> MDPPRPALLALLALPALLLLLLAGARAEEEMLENVSLVCPKDATRFKHLRKYTYNYEAESSSGVPGTADSRSATRINCKVELEVPQLCSFILKTSQCTLKEVYGFNPEGKALLKKTKNSEEFAAAMSRYELKLAIPEGKQVFLYPEKDEPTYILNIKRGIISALLVPPETEEAKQVLFLDTVYGNCSTHFTVKTRKGNVATEISTERDLGQCDRFKPIRTGISPLALIKGMTRPLSTLISSSQSCQYTLDAKRKHVAEAICKEQHLFLPFSYKNKYGMVAQVTQTLKLEDTPKINSRFFGEGTKKMGLAFESTKSTSPPKQAEAVLKTLQELKKLTISEQNIQRANLFNKLVTELRGLSDEAVTSLLPQLIEVSSPITLQALVQCGQPQCSTHILQWLKRVH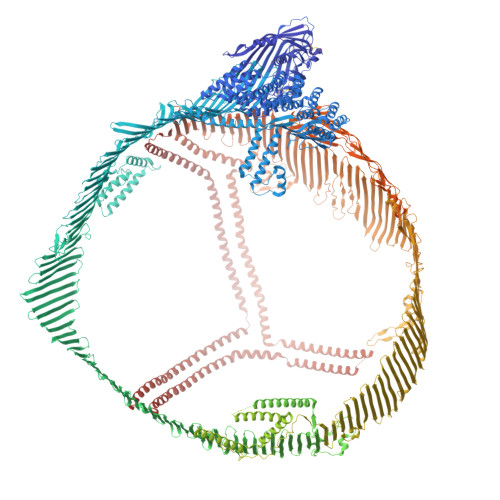ANPLLIDVVTYLVALIPEPSAQQLREIFNMARDQRSRATLYALSHAVNNYHKTNPTGTQELLDIANYLMEQIQDDCTGDEDYTYLILRVIGNMGQTMEQLTPELKSSILKCVQSTKPSLMIQKAAIQALRKMEPKDKDQEVLLQTFLDDASPGDKRLAAYLMLMRSPSQADINKIVQILPWEQNEQVKNFVASHIANILNSEELDIQDLKKLVKEALKESQLPTVMDFRKFSRNYQLYKSVSLPSLDPASAKIEGNLIFDPNNYLPKESMLKTTLTAFGFASADLIEIGLEGKGFEPTLEALFGKQGFFPDSVNKALYWVNGQVPDGVSKVLVDHFGYTKDDKHEQDMVNGIMLSVEKLIKDLKSKEVPEARAYLRILGEELGFASLHDLQLLGKLLLMGARTLQGIPQMIGEVIRKGSKNDFFLHYIFMENAFELPTGAGLQLQISSSGVIAPGAKAGVKLEVANMQAELVAKPSVSVEFVTNMGIIIPDFARSGVQMNTNFFHESGLEAHVALKAGKLKFIIPSPKRPVKLLSGGNTLHLVSTTKTEVIPPLIENRQSWSVCKQVFPGLNYCTSGAYSNASSTDSASYYPLTGDTRLELELRPTGEIEQYSVSATYELQREDRALVDTLKFVTQAEGAKQTEATMTFKYNRQSMTLSSEVQIPDFDVDLGTILRVNDESTEGKTSYRLTLDIQNKKITEVALMGHLSCDTKEERKIKGVISIPRLQAEARSEILAHWSPAKLLLQMDSSATAYGSTVSKRVAWHYDEEKIEFEWNTGTNVDTKKMTSNFPVDLSDYPKSLHMYANRLLDHRVPQTDMTFRHVGSKLIVAMSSWLQKASGSLPYTQTLQDHLNSLKEFNLQNMGLPDFHIPENLFLKSDGRVKYTLNKNSLKIEIPLPFGGKSSRDLKMLETVRTPALHFKSVGFHLPSREFQVPTFTIPKLYQLQVPLLGVLDLSTNVYSNLYNWSASYSGGNTSTDHFSLRARYHMKADSVVDLLSYNVQGSGETTYDHKNTFTLSCDGSLRHKFLDSNIKFSHVEKLGNNPVSKGLLIFDASSSWGPQMSASVHLDSKKKQHLFVKEVKIDGQFRVSSFYAKGTYGLSCQRDPNTGRLNGESNLRFNSSYLQGTNQITGRYEDGTLSLTSTSDLQSGIIKNTASLKYENYELTLKSDTNGKYKNFATSNKMDMTFSKQNALLRSEYQADYESLRFFSLLSGSLNSHGLELNADILGTDKINSGAHKATLRIGQDGISTSATTNLKCSLLVLENELNAELGLSGASMKLTTNGRFREHNAKFSLDGKAALTELSLGSAYQAMILGVDSKNIFNFKVSQEGLKLSNDMMGSYAEMKFDHTNSLNIAGLSLDFSSKLDNIYSSDKFYKQTVNLQLQPYSLVTTLNSDLKYNALDLTNNGKLRLEPLKLHVAGNLKGAYQNNEIKHIYAISSAALSASYKADTVAKVQGVEFSHRLNTDIAGLASAIDMSTNYNSDSLHFSNVFRSVMAPFTMTIDAHTNGNGKLALWGEHTGQLYSKFLLKAEPLAFTFSHDYKGSTSHHLVSRKSISAALEHKVSALLTPAEQTGTWKLKTQFNNNEYSQDLDAYNTKDKIGVELTGRTLADLTLLDSPIKVPLLLSEPINIIDALEMRDAVEKPQEFTIVAFVKYDKNQDVHSINLPFFETLQEYFERNRQTIIVVLENVQRNLKHINIDQFVRKYRAALGKLPQQANDYLNSFNWERQVSHAKEKLTALTKKYRITENDIQIALDDAKINFNEKLSQLQTYMIQFDQYIKDSYDLHDLKIAIANIIDEIIEKLKSLDEHYHIRVNLVKTIHDLHLFIENIDFNKSGSSTASWIQNVDTKYQIRIQIQEKLQQLKRHIQNIDIQHLAGKLKQHIEAIDVRVLLDQLGTTISFERINDILEHVKHFVINLIGDFEVAEKINAFRAKVHELIERYEVDQQIQVLMDKLVELAHQYKLKETIQKLSNVLQQVKIKDYFEKLVGFIDDAVKKLNELSFKTFIEDVNKFLDMLIKKLKSFDYHQFVDETNDKIREVTQRLNGEIQALELPQKAEALKLFLEETKATVAVYLESLQDTKITLIINWLQEALSSASLAHMKAKFRETLEDTRDRMYQMDIQQELQRYLSLVGQVYSTLVTYISDWWTLAAKNLTDFAEQYSIQDWAKRMKALVEQGFTVPEIKTILGTMPAFEVSLQALQKATFQTPDFIVPLTDLRIPSVQINFKDLKNIKIPSRFSTPEFTILNTFHIPSFTIDFVEMKVKIIRTIDQMLNSELQWPVPDIYLRDLKVEDIPLARITLPDFRLPEIAIPEFIIPTLNLNDFQVPDLHIPEFQLPHISHTIEVPTFGKLYSILKIQSPLFTLDANADIGNGTTSANEAGIAASITAKGESKLEVLNFDFQANAQLSNPKINPLALKESVKFSSKYLRTEHGSEMLFFGNAIEGKSNTVASLHTEKNTLELSNGVIVKINNQLTLDSNTKYFHKLNIPKLDFSSQADLRNEIKTLLKAGHIAWTSSGKGSWKWACPRFSDEGTHESQISFTIEGPLTSFGLSNKINSKHLRVNQNLVYESGSLNFSKLEIQSQVDSQHVGHSVLTAKGMALFGEGKAEFTGRHDAHLNGKVIGTLKNSLFFSAQPFEITASTNNEGNLKVRFPLRLTGKIDFLNNYALFLSPSAQQASWQVSARFNQYKYNQNFSAGNNENIMEAHVGINGEANLDFLNIPLTIPEMRLPYTIITTPPLKDFSLWEKTGLKEFLKTTKQSFDLSVKAQYKKNKHRHSITNPLAVLCEFISQSIKSFDRHFEKNRNNALDFVTKSYNETKIKFDKYKAEKSHDELPRTFQIPGYTVPVVNVEVSPFTIEMSAFGYVFPKAVSMPSFSILGSDVRVPSYTLILPSLELPVLHVPRNLKLSLPDFKELCTISHIFIPAMGNITYDFSFKSSVITLNTNAELFNQSDIVAHLLSSSSSVIDALQYKLEGTTRLTRKRGLKLATALSLSNKFVEGSHNSTVSLTTKNMEVSVATTTKAQIPILRMNFKQELNGNTKSKPTVSSSMEFKYDFNSSMLYSTAKGAVDHKLSLESLTSYFSIESSTKGDVKGSVLSREYSGTIASEANTYLNSKSTRSSVKLQGTSKIDDIWNLEVKENFAGEATLQRIYSLWEHSTKNHLQLEGLFFTNGEHTSKATLELSPWQMSALVQVHASQPSSFHDFPDLGQEVALNANTKNQKIRWKNEVRIHSGSFQSQVELSNDQEKAHLDIAGSLEGHLRFLKNIILPVYDKSLWDFLKLDVTTSIGRRQHLRVSTAFVYTKNPNGYSFSIPVKVLADKFIIPGLKLNDLNSVLVMPTFHVPFTDLQVPSCKLDFREIQIYKKLRTSSFALNLPTLPEVKFPEVDVLTKYSQPEDSLIPFFEITVPESQLTVSQFTLPKSVSDGIAALDLNAVANKIADFELPTIIVPEQTIEIPSIKFSVPAGIVIPSFQALTARFEVDSPVYNATWSASLKNKADYVETVLDSTCSSTVQFLEYELNVLGTHKIEDGTLASKTKGTFAHRDFSAEYEEDGKYEGLQEWEGKAHLNIKSPAFTDLHLRYQKDKKGISTSAASPAVGTVGMDMDEDDDFSKWNFYYSPQSSPDKKLTIFKTELRVRESDEETQIKVNWEEEAASGLLTSLKDNVPKATGVLYDYVNKYHWEHTGLTLREVSSKLRRNLQNNAEWVYQGAIRQIDDIDVRFQKAASGTTGTYQEWKDKAQNLYQELLTQEGQASFQGLKDNVFDGLVRVTQEFHMKVKHLIDSLIDFLNFPRFQFPGKPGIYTREELCTMFIREVGTVLSQVYSKVHNGSEILFSYFQDLVITLPFELRKHKLIDVISMYRELLKDLSKEAQEVFKAIQSLKTTEVLRNLQDLLQFIFQLIEDNIKQLKEMKFTYLINYIQDEINTIFSDYIPYVFKLLKENLCLNLHKFNEFIQNELQEASQELQQIHQYIMALREEYFDPSIVGWTVKYYELEEKIVSLIKNLLVALKDFHSEYIVSASNFTSQLSSQVEQFLHRNIQEYLSILTDPDGKGKEKIAELSATAQEIIKSQAIATKKIISDYHQQFRYKLQDFSDQLSDYYEKFIAESKRLIDLSIQNYHTFLIYITELLKKLQSTTVMNPYMKLAPGELTIIL>GPLGSMKQMGSMHPVQVIAVTGGKGGVGKTNVSVNLALALADLGRRVMLLDADLGLANVDVLLGLTPKRTLADVIEGRCELRDVLLLGPGGVRIVPAASGTQSMVHLSPMQHAGLIQAFSDISDNLDVLVVDTAAGIGDSVVSFVRAAQEVLLVVCDEPTSITDAYALIKLLNRDHGMTRFRVLANMAHSPQEGRNLFAKLTKVTDRFLDVALQYVGVIPYDESVRKAVQKQRAVYEAFPRSKASLAFKAVAQKVDSWPLPANPRGHLEFFVERLVQHP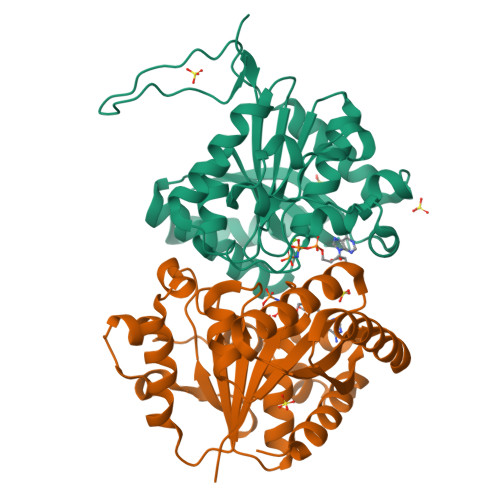ATGSAV[2x]>RGSHHHHHHG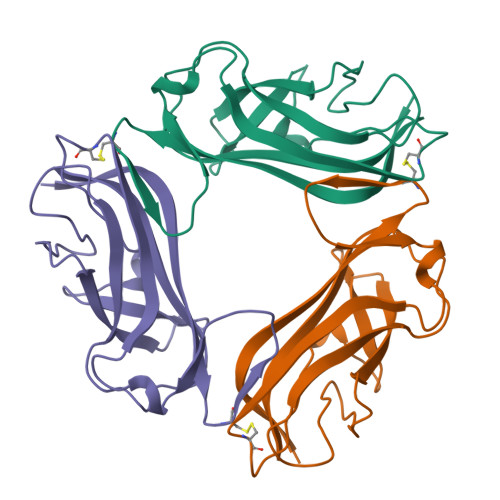SFTPSGTTGTTKLTVTEECQVRVGDLTVAKTRGQLTDAAPIGPVTVQALGCNARQVALKADTDNFEQGKFFLISDNNRDKLYVNIRPMDNSAWTTDNGVFYKNDVGSWGGTIGIYVDGQQTNTPPGNYTLTLTGGYWAK[9x]>[12x]AECSVDIQGNDQMQFNTNAITVDKSCKQFTVNLSHPGNLPKNVMGHNWVLSTAADMQGVVTDGMASGLD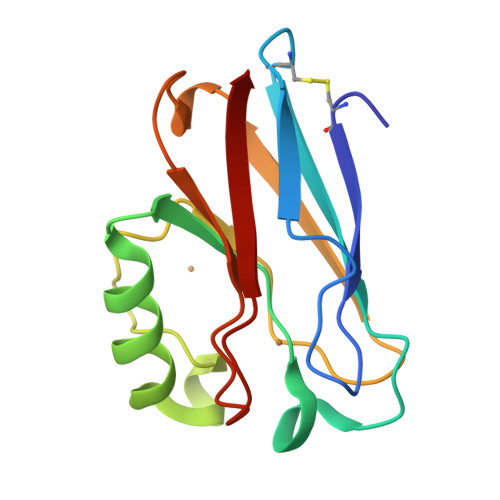KDYLKPDDSRVIAHTKLIGSGEKDSVTFDVSKLKEGEQYMFFCTFPGGSALMKGTLTLK> GGEETAAPASDFDDKVTVGILHSLTGTMAISESTLVDTEKMAIDEINAAGGVEVDGKKYKIEYIVEDGASDWPTFAEKSKKLIDQDQVPVVFGGWTSASRKAMLPVYESKNAFLYYPIQYEGQECSNNIFYTGATPNQQSEPATKFMYEKSPAAGKPFFLVGSDYVFPRTSNTITKEQLASLGGEVVGEDYLPLGNTEVAPIIAKIKKALPDGGVIINTLNGDQNVAFFKQIQDAGITPDNGYYVMSYSIAEEEISTIGSEFLEGHYGAWNYMMSIDTPASKKFAADFKAKYGADRQVADPQESAYNMVYLWKKAV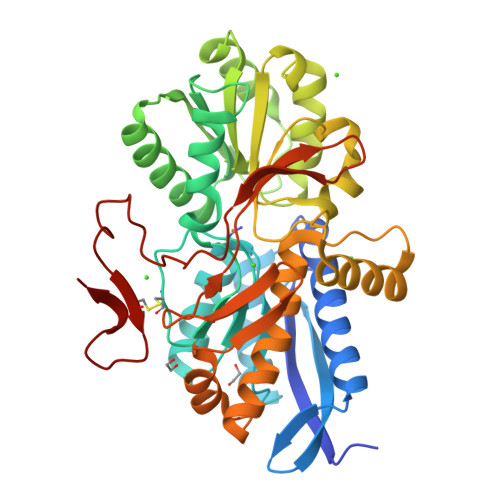EKANSFDDDKVREVLVGIEFDAPQGPVKVMPNHHLSQTVRIGQITADGQFEILESTDGPVAPQAWNQFEPSSKGFACDWTDAAKGEKYKL> SHHHHHHSSSENLYFQSMESMPNAVELTVENAWFIAEMVGAGTFPWVLAITTPYSDEAQRSAFFARQRDELTQLGLLSSDGVVNPAVAEWIKVVCFPERWLDLRYVGPGTGNGGEDLLRGIVAQSAGIMGKAGKAHPSFNTVVALRNAQLVTFTAMDIDDPRALVPVLGVGLSARPPARFEEFSMPMRVGARADERLRSGESLDEVLDYLGIPVSARPVVQAVFSGPRSYVEIVAGCNRDGEHTT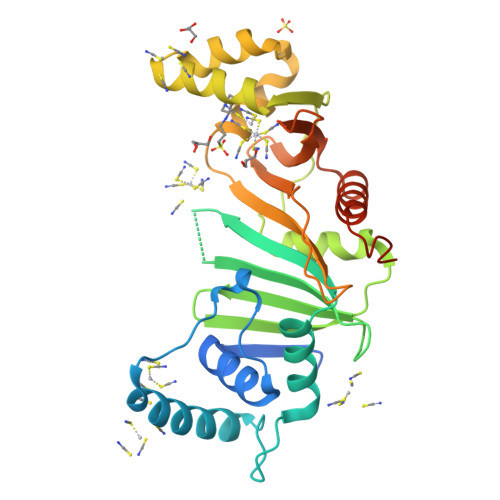TDVGLSIVDTTAGRVLVSPSRAFDGEWVSTFSAGTPFATAVAIDQLIANLPDGQWFPGQRLSRDFSSQPS> MSSGHHHHHHSYRVSTGAAHAAKGGGLVSGDSYSMMELGARKYAIAISDGMGNGARAHFESNETIKLLEKILESGIDEKIAIKTINSILSLRTTDEIYSTLDLSIIDLQDASCKFLKVGSTPSFIKRGDQVMKVQASNLPIGIINEFDVEVVSEQLKAGDLLIMMSDGIFEGPKHVENHDLWMKRKMKGLKTNDPQEIADLLMEEVIRTRSGQIEDDMTVVVVRIDHNTPKWASIPVPAIFQNKQEIS

We investigated the PP2C family member SpoIIE, which controls the activation of the cell-specific transcription factor σF during the developmental process of sporulation in the bacterium Bacillus subtilis. SpoIIE is the most upstream member of a three-protein pathway that activates σF in the small cell. It does so by dephosphorylating the phosphoprotein SpoIIAA-P. Dephosphorylated SpoIIAA, in turn, displaces σF from the anti-sigma factor SpoIIAB to release the free and active transcription factor. Like other PP2C family phosphatases, the catalytic center of SpoIIE uses two divalent cations (manganese in the case of SpoIIE) to deprotonate a water molecule that serves as the nucleophile for dephosphorylation.

Previously, we determined the structure of SpoIIE590–827, a fragment that included the PP2C phosphatase domain but lacked the adjacent regulatory domain. Although monomeric in solution under physiological conditions, SpoIIE590–827 had undergone a domain-swap dimerization during crystallization. Here, we solved an additional structure for SpoIIE590–827 (with an amino acid substitution A624I that was designed to block domain swapping) that was in a different crystal form and was not domain-swapped. Importantly, the only significant differences between the two SpoIIE590–827 structures were at the site of the domain-swap. We hypothesized that this structure represented the inactive state because it lacked the dimeric interface of the SpoIIE457–827 structure. Comparison of the SpoIIE590–827 structures with SpoIIE457–827 revealed that dimerization rotated the switch helices (α1 and α2 of the PP2C fold, corresponding to SpoIIE residues 630–678) approximately 45° as a rigid body relative to the phosphatase core. Our structure of SpoIIE590–827 reveals that in the monomeric state, V697 packs in a hydrophobic pocket between the β strands at the base of the PP2C domain and the switch. Based on the universally conserved architecture of the catalytic center, the M2 metal of SpoIIE is predicted to be coordinated by the side-chain of D628 and the carbonyl oxygen of G629. G629 is at the junction between the switch helices and the β strands at the base of the phosphatase domain, such that movement of the switch helices could be coupled with bringing G629 into position to recruit M2. In support of this idea, G629 is not in position to coordinate M2 in our isolated phosphatase domain structures, which we thus conclude represent an inactive state.> SPNVEACGYSDRVRQITLGNSTITTQEAANAIVAYGEWPTYINDSEANPVDAPTEPDVSSNRFYTLESVSWKTTSRGWWWKLPDCLKDMGMFGQNMYYHYLGRSGYTIHVQCNASKFHQGALGVFLIPEFVMACNTESKTSYVSYINANPGERGGEFTNTYNPSNTDASEGRKFAALDYLLGSGVLAGNAFVYPHQIINLRTNNSATIVVPYVNSLVIDCMAKHNNWGIVILPL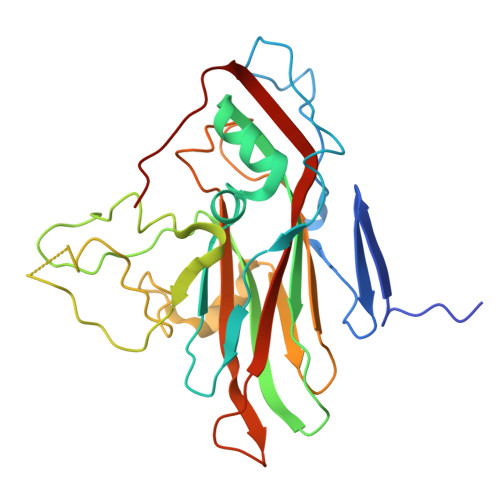APLAFAATSSPQVPITVTIAPMCTEFNGLRNITVPVHQ> EPLRVLELYSGVGGMHHALRESCIPAQVVAAIDVNTVANEVYKYNFPHTQLLAKTIEGITLEEFDRLSFDMILMSPPCQPFTRIGRQGDMTDSRTNSFLHILDILPRLQKLPKYILLENVKGFEVSSTRDLLIQTIENCGFQYQEFLLSPTSLGIPNSRLRYFLIAKLQSEPLPFQAPGQVLMEFPKIEIHRKNQQDSDLSVKMLKDFLEDDTDVNQYLLPPKSLLRYALLLDIVQPTCRRSVCFTKGYGSYIE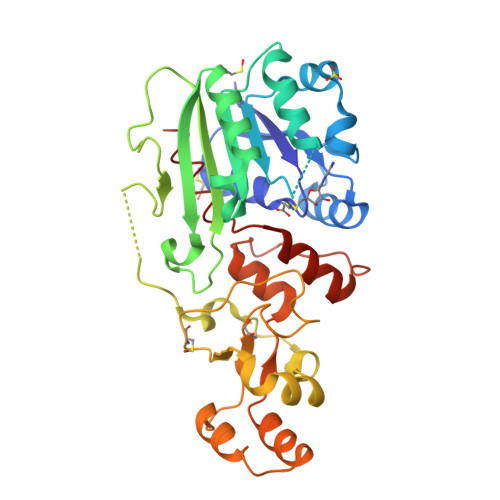GTGSVLQTAEDVQVENIYKSLTNLSQEEQITKLLILKLRYFTPKEIANLLGFPPEFGFPEKITVKQRYRLLGNSLNVHVVAKLIKILYE>[2x]CPRFLKVKNWETDVVLTDTLHL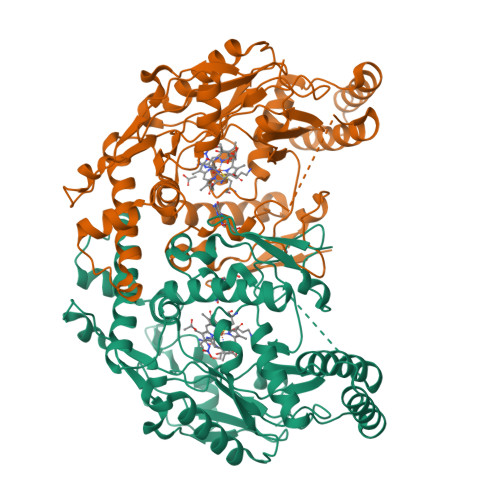KSTLETGCTEHICMGSIMLPSQHTRKPEDVRTKDQLFPLAKEFLDQYYSSIKRFGSKAHMDRLEEVNKEIESTSTYQLKDTELIYGAKHAWRNASRCVGRIQWSKLQVFDARDCTTAHGMFNYICNHVKYATNKGNLRSAITIFPQRTDGKHDFRVWNSQLIRYAGYKQPDGSTLGDPANVQFTEICIQQGWKAPRGRFDVLPLLLQANGNDPELFQIPPELVLEVPIRHPKFDWFKDLGLKWYGLPAVSNMLLEIGGLEFSACPFSGWYMGTEIGVRDYCDNSRYNILEEVAKKMDLDMRKTSSLWKDQALVEINIAVLYSFQSDKVTIVDHHSATESFIKHMENEYRCRGGCPADWVWIVPPMSGSITPVFHQEMLNYRLTPSFEYQPDPWNTHVWK> GMSQDKWLEWAVRLQALAQTGLAYGKDVYDMERFEEIRQIAAEMLVEPSGQPLEVVKDLFCNETGYQTPKLDTRAAIFQEDKILLVQENDGLWSLPGGWCDVDQSVKDNVVKEVKEEAGLDVEAQRVVAILDKHKNNPAKSAHRVTKVFILCRLLGGEFQPNSETVASGFFSLDDLPPLYLGKNTAEQLALCLEASRSEHW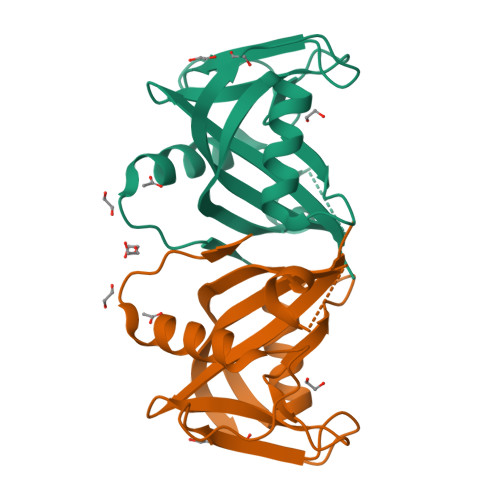ETRFD>MSTPAPPEEQARLLEDALIAVRQQTAMMRKFLDTPGKLMDALKCCSTLVSELRTSSLSPKQYYELYMAVFDALRYLSAHLRENHPVNHLADLYELVQYAGNIIPRLYLMITVGTAYMSIDGAPVKELMKDMMDMSRGVQHPVRGLFLRYYLSGQARDYLPTGDSDGPEGNLQDSINFILTNFVEMNKLWVRLQHQGHSRERDLRTQERRELQLLVGSNIVRLSQLVDLPTYRDSILGPLLEQIVQCRDILAQEYLLEVITQVFPDEYHLHTLDQFLGAVSRLNPHVNVKAIVIGMMNRLSDYAERESQNEPEEDRAKLEEEALAKLLEKTKLGQNSELEPQNGDHPDTEVSSTTDSAQAPSTADSDTTAVNGEEEPVRKRRGIPVNVPLYDIFFDQVQHLVQAQHLPIQDTIALCCSLANLSLNIYPERLDYVDGILAYALAKVKEHANSADLHSQPAQQSLLSLLQSPLRRYVSIFTALSLPTYVSLFQAQTYPTRRAIAGEIVRTLLKNQTLISTPAHLENVLEILKVLIKEGSQPPAGYPGVVQPRARPLETDETMEEQGWLARLVHLIHSDDNDTQFRLLQMTRKAYAEGNERIRTTTPPLITAGLKLARRFKAREHYDDNWSSQSSSLFKFLHSAISTLYTRVNGPGVADLCLRLFCSCGQVADMTEFEEVAYEFFAQAFTVYEESISDSKAQFQAVCVIASALHRTRNFGRENYDTLITKCAQHASKLLRKPDQCRAVYLASHLWWATPIAARGETEDTELYRDGKRVLECLQRALRVADSCMETATSIELFVEILDRYVYYFDQR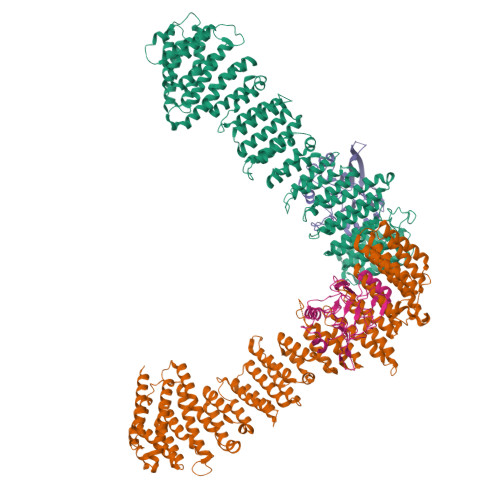NESVTTKYLNGLIELIHSNLAGNQQDSASVEASRKHFIQTLEMIQSKEFEGIVVAPK[2x];>SMAFLILVIGNLHIPDRALDIPPKFKKLLSPGKISQTLCLGNLTDRATYDYLRSISPDLKIVRGRMDVEATSLPLMQVVTHGSLRIGFLEGFTLVSEEPDVLLAEANKLDVDVLCWAGGSHRFECFEYMDKFFVNPGSATGAFTTDWLAEGEEVVPSFCLMDVQGISLTLYVYQLRKDENGTENVAVEKVTYTKPVEPTGAS[2x]> SIQVTPRSIVINRMNNIQINPTSIGNPNNGLHMTYNNAAAAAAAAAAAAAAAAAAAAAAAAAAAAAAAASIQVTPRSIVINRMNNIQINPTSIGNPQVTIRLPLNNFKSTTQLIQQVSLTDFFRPDIEHAGSTVLILRHPTDLPALARHRAPPGRQTERLAEAWGQLLEASRAYVTSLSFIAACRAEEYTDKQAAEANRTAIVSAYGCSRMGARLIRFSECLRAMVQCHVFPHRFISFFGSLLEYTIQDNLCNITAVAKGPQEAARTDKTSTRRVTANIPACVFWDVDKDLHLSADGLKHVFLVFV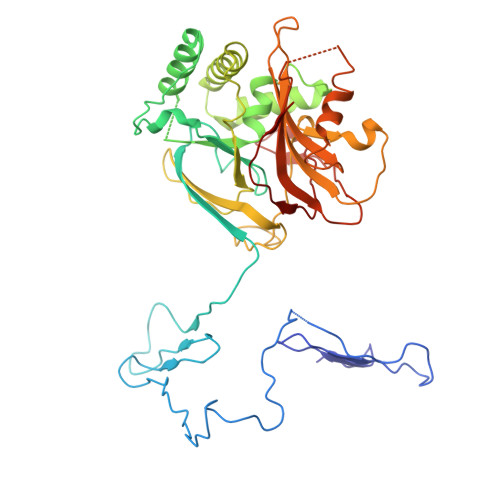YTQRRQREGVRLHLALSQLNEQCFGRGIGFLLGARICMYAAYTLIGTIPSESVRYTRRMERFGGYNVPTIWLEGVVWGGTNTWNEC> MSEMTPREIVSELDQHIIGQADAKRAVAIALRNRWRRMQLQEPLRHEVTPKNILMIGPTGVGKTEIARRLAKLANAPFIKVEATKFTEVGYVGKEVDSIIRDLTDSAMKLVRQQEIAKNRARAEDVAEERILDALLPPAKNQWGEVENHDSHSSTRQAFRKKLREGQLDDKEIEIDVSAGVSMGVEIMAPPGMEEMTNQLQSLFQNLGSDKTKKRKMKIKDALKALIDDEAAKLINPEELKQKAIDAVEQNGIVFIDEIDKICKKGEYSGADVSREGVQRDLLPLVEGSTVSTKHGMVKTDHILFIASGAFQVARPSDLIPELQGRLPIRVELTALSAADFERILTEPHASLTEQYKALMATEGVNIAFTTDAVKKIAEAAFRVN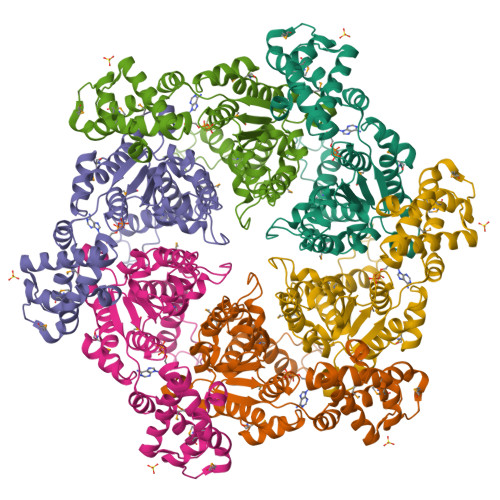EKTENIGARRLHTVMERLMDKISFSASDMNGQTVNIDAAYVADALGEVVENEDLSRFIL>[10x]SAMDLPDVTLSLCGGLSENGEISKEKFMEHIITYHEFAENPGLIDNPNLVIRIYNRYYNWALAAPMILSLQVFQKSLPKATVESWVKDKMP

Lipins are magnesium-dependent phosphatidic acid phosphatases (PAPs) that catalyze the dephosphorylation of the membrane lipid phosphatidic acid (PA) to produce diacylglycerol (DAG). Our principal findings are that the M-Lip domain is a new protein fold that forms a dimer, binds membranes, and can affect lipin PAP activity, oligomerization, subcellular localization, and adipogenesis. Phospholipid synthesis and fat storage as triglycerides are regulated by lipin phosphatidic acid phosphatases (PAPs), whose enzymatic PAP function requires association with cellular membranes.

We also determined the structure of the mouse lipin 2 M-Lipxtal domain to 2.5 Å resolution. The M-Lip domain of mouse lipin 1 and lipin 2 formed a symmetric or near symmetric dimer in all three crystal forms with a root mean square deviation for all atoms ranging between 0.36–0.77 Å. The observation of near identical dimers in three different crystal structures strongly suggested the native quaternary structure of the M-Lip domain as dimeric. Notably, the residues involved in dimerization were highly conserved among human and mouse lipin 1, lipin 2, and lipin 3 paralogs. Lastly, our data suggest that the conserved dimer interface of the M-Lip may contribute to both homo and hetero-dimerization of mammalian lipins.>[2x]SGSME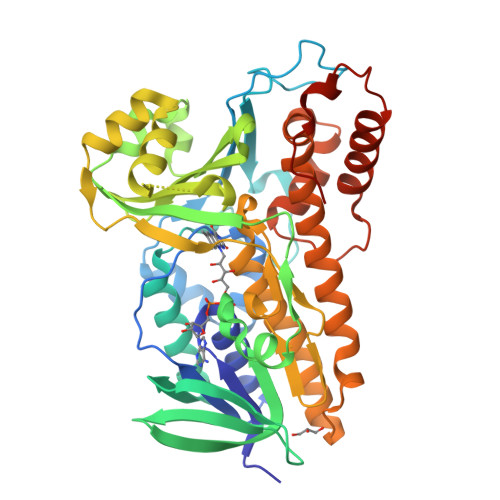PQFDVGIIGGGPAGSTTASYLARAGLKVALFESDNFPREHVGESLVPATTPVLVDIDAFDKVEAAGFPKKFGAAWTSADSGPSDKMGFTGLDHDFRAAEIMFNERTQSGVHKDYTFHVDRGQFDLLLLKHAEEQGAKVHQGVRVNRVNFDGAFPVLETSVAGQRAKVPVKMVVDASGRRTQLGSQLKVKEKDPVFNQYAIHTWFDNFDRKALAVDQSQSDFIFIHFLPVIDTWVWQIPITDTITSVGVVTQKERLKASKDDLEKFFWDTLGSRPELHKALKESEQVRPLKTEGDYSYALTKVCGDNFLMVGDAARFVDPIFSSGVSVALNSARIASADIIAAHRAGDYSKKRFDTYESMLRRGVNNWYEFISIYYRLNILFTAFVQDPRYRIDVLKMLQGDVYDDEEPKALAAMREIVKAVEEDPNHLWHPFLGSLKAPSAKAMF> GPLGSMASITQLFDDLCEALLPAAKTHLGQRSVNRKRAKRSLKKVAYNALFTNLFQDETQQLQPDMSKLPARNKILMLSF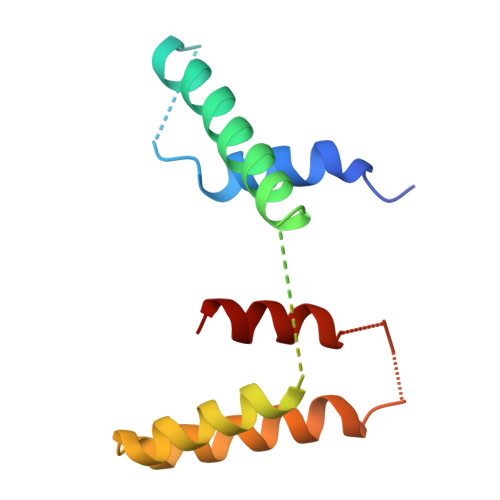DLRVGGLGPKADRLEELVEELEAAPCCPLLEVGSVLDLLVQLAG> MAHHHHHHMMNKDKNKRVISAPRGTEIQAKNWLTEAALRMICNNLDPNVAEDPDSLIVYGGLGKAARNWECFDEIVHVLKLLNNDQTLLIQSGKPVGVFTTHEEAPRILIANSNLVPRWATWEHFNELDKKGLMMYGQMTAGSWIYIGSQGIVQGTYETFVAAAKKHYQGDLSGRWILTAGLGGMGGAQPLAGTMAGASVLAVECDRQRIEKRLQTKYLDRYTDNLSEALDWINESCRRKKPVSVAVLGNAAEIFPQLVKLGVQPSLVTDQTS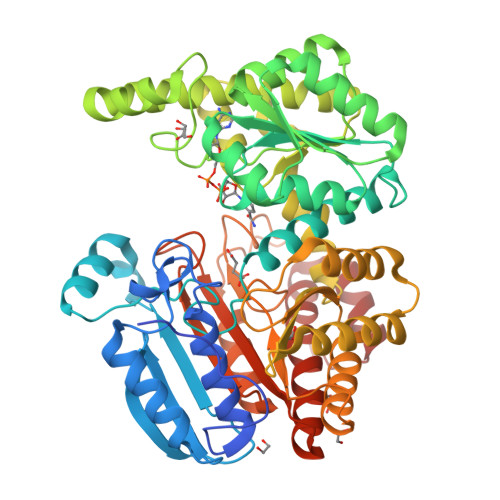AHDPLNGYLPLGWTLEQAVEMRKKSPEEVVDAAKKSMAVQVHAMLEFHNRGIPVFDYGNNIRQMAFEAGEKNAFSFEGFVPAYIRPLFCEGIGPFRWVALSGDPEDIYATDERVKQLIPDAPHLHHWLDMAREKISFQGLPARICWVGLKDRARLALAFNEMVKNKQVKAPIVIGRDHLDSGSVASPNRETEGMLDGSDAVSDWPLLNALLNCASGATWVSIHHGGGVGMGFSQHAGVVIVADGTEKAAKRLARVLHNDPATGVMRHADAGYQIAKQCAKENSLWLPMES> MGSDKIHHHHHHMNVINETANVLKLETGSVTSAKGFSAVGIHTGVKRKRKDLGAIVCEVPASSAAVYTLNKVQAAPLKVTQESIAVEGKLQAMIVNSGIANACTGKRGLDDAYTMRAVGAETFHIPEHYVAVTSTGVIGEFLPMDVITN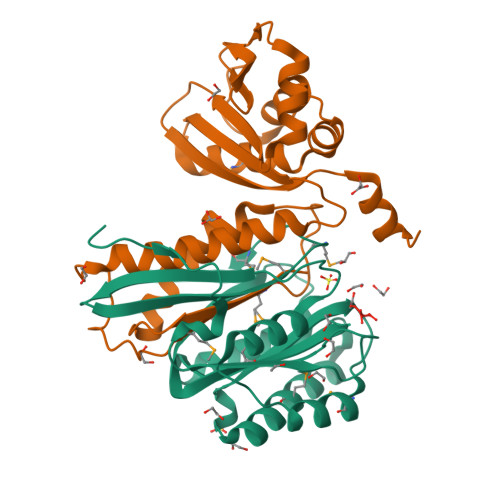GIRQLKPEATIEGAHAFNEAILTTDTVEKHTCYQTIVNGKTVTVGGVAKGSGMIHPNMA;> TMLSFVTTDANIDHGHLQGALSAITNETFNRITVDGDTSTNDMVVVMASGLAENETLTPEHPDWANFYKALQLACEDLAKQIARDGEGATKLIEVEVTGAANDQEAGMVAKQIVGSDLVKTAIYGADANWGRIICAIGYSGCEVNQETIDIAIGPIVTLKQSEPTGFSEEEATAYLKEADPVKISVNLHIGNGTGKAWGCDLTYDYVRINAGYRT>[2x]MDVARNGARGSVESPPNRKVYMDYNATTPLEPEVIQAVTEAMKEAWGNPSSSYVAGRKAKDIINTARASLAKMIGGKPQDIIFTSGGTESNNLVIHSTVRCFHEQQTLQGRTVDQISPEEGTRPHFI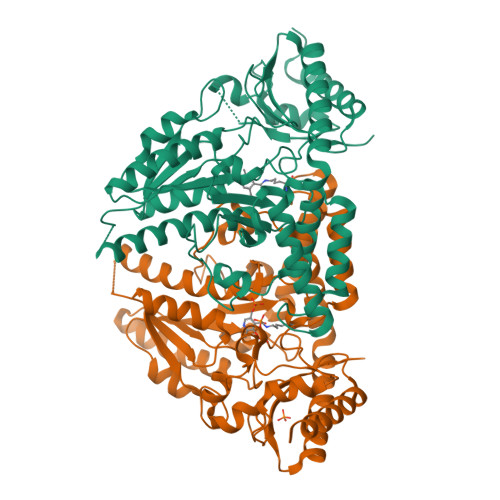TCTVEHDSIRLPLEHLVEDQVAEVTFVPVSKVNGQVEVEDILAAVRPTTCLVTIMLANNETGVIMPISEISRRIKALNQIRAASGLPRVLVHTDAAQALGKRRVDVEDLGVDFLTIVGHKFYGPRIGALYVRGVGKLTPLYPMLFGGGQERNFRPGTENTPMIAGLGKAADLVSENCETYEAHMRDIRDYLEERLEAEFGKRIHLNSRFPGVERLPNTCNFSIQGSQLRGYMVLAQCQTLLASVGASCHSDHEDRPSPVLLSCGIPVDVARNAVRLSVGRSTTRAEVDLIVQDLKQAVNQLEGPV>[2x]GSMKLFAQGTSLDLSHPHVMGILNVTPDSFSDGGTHNSLIDAVKHANLMINAGATIIDVGGESTRPGAAEVSVEEELQRVIPVVEAIAQRFEVWISVDTSKPEVIRESAKVGAHIINDIRSLSEPGALEAAAETGLPVCLMHMQGNPKTMQEAPKYDDVFAEVNRYFIEQIARCEQAGIAKEKLLLDPGFGFGKNLSHNYSLLARLAEFHHFN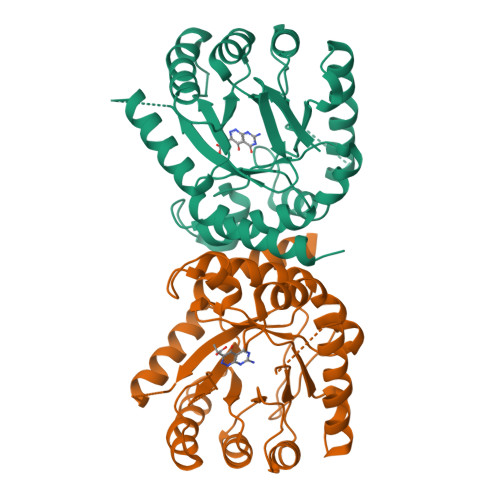LPLLVGMSRKSMIGQLLNVGPSERLSGSLACAVIAAMQGAHIIRVHDVKETVEAMRVVEATLSAKENKRYE>AAPALKEIFNV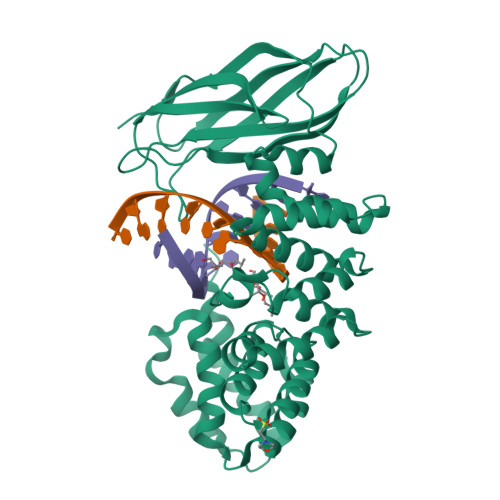ERLQHIASEMTAVYPAFDAKGFLKHAKAGLAELSVMQRMARVSESLHAVIPLDYPQTLTLLYALAPRLNSGFVSLFLPHYVASYGRDDFKRSMAALKYFTTFGSAEFAIRHFLLHDFQRTLAVMQAWSQDDNEHVRRLASEGSRPRLPWSFRLAEVQADPELCASILDHLKADSSLYVRKSVANHLNDITKDHPEWVLSLIEGWNLENPHTAWIARHALRSLIKQGNTRALTLMGAGAKAEVKIHHLMVTPAVINLGERINLSFTLESTAPAPQKLVVDYAIDYVKSTGHGAAKVFKLKAFSLGAGAQQHIRREQHIRDMTTRKHYPGRHVVHVLVNGERLGSAEFELRA[2x]> MTNSDDDLFSE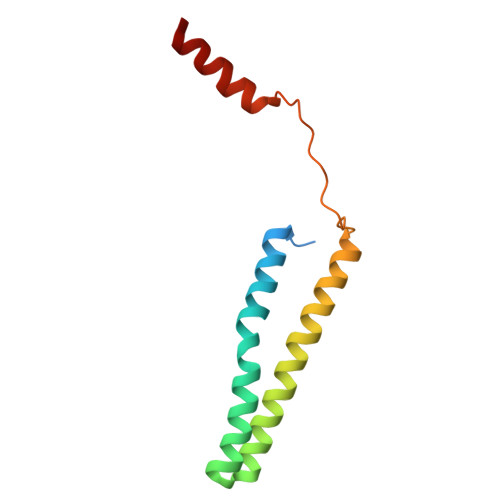KSTSSDTQQVQNILELEAKIPDILSSAGKCIEAIQLNNSLEDFRKYSKEFLETVEFISTGLRRQALELEKAEVPVVSLQPKKRYASTPLSNLIFDQSSKLM methyl 2-(4-cyanophenoxy)ethanoate 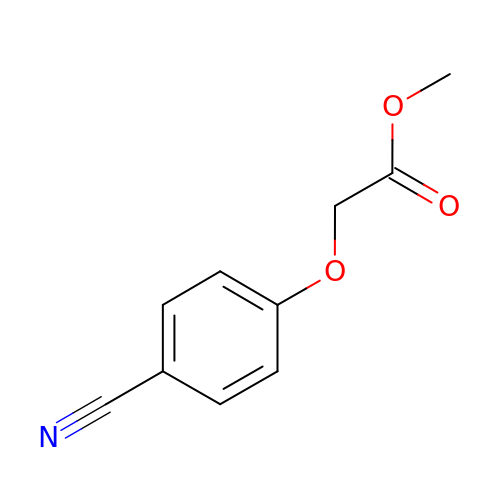| C10 H9 N O3 | MAVSETCJUQQWBN-UHFFFAOYSA-N STAT6 becomes activated in response to IL-4 and IL-13 and mediates most of the gene expression regulated by these cytokines. By direct interaction with specific parts of its transactivation domain, STAT6 recruits the co-activators p300/CBP and NCoA1 (also called steroid receptor coactivator-1, SRC-1), which are essential for transcriptional activation. In particular, the interaction between STAT6 and NCoA1 is modulated by a short region of the transactivation domain that includes the motif LXXLL (where L is leucine and X is any amino acid). Here, we report the structural characterization of the complex between a STAT6-derived peptide encompassing the region from Gly783 to Gly814 and the NCoA1 PAS-B domain257–385 using NMR and X-ray crystallography.

In this crystal structure the residues located in the N-terminal part (Gly783 - Pro793) are not ordered indicating that this region is too dynamic to be resolved in the crystal. Nevertheless, the new X-ray structure of the complex clarifies the structural role of Leu794 whose side chain fits into a deep pocket on the cofactor surface formed by Phe314, Phe300 and Ala310. Yet, there is no interaction visible between the residues N-terminal of Leu794 in the crystal structure. Therefore, we decided to perform a structural characterization of the NCoA1257–385/STAT6783–814 complex by NMR. Importantly, the interaction between the NCoA1 PAS-B domain and STAT6783–814 is further stabilized by the interaction of STAT6 Leu794 with a shallow hydrophobic indentation constituted by the PAS-B domain residues Phe314, Phe300 and Ala310, seen also in the X-ray structure and in agreement with the alanine scanning mutagenesis data where F794A reduced the affinity about 50-fold. In addition, the two isoleucine residues (Ile786, Ile790) located in the N-terminal part of the STAT6 peptide bind into a shallow hydrophobic pocket on the surface of the PAS-B domain formed by Phe314, Met318, Leu346, Pro356 and Ile358. The NMR structure of the NCoA1257–385/STAT6783–814 complex indicates that the coactivator recognition mechanism by STAT6 occurs by the formation of a partially ordered complex in which two α-helical regions (Ile786-Ile790 and Glu799-Glu808) are connected by a linker that adopts an extended, albeit dynamic, conformation. This dynamics in the linker may act more strongly onto the N-terminal region of the STAT6783–814 peptide that has fewer interactions with the NcoA1 PAS-B domain than the C-terminal region, ultimately rendering residues 783–793 disordered in the X-ray structure. Thus despite the invisibility of the peptide N-terminal to Leu794 in the X-ray structure, the complex formation between the NCoA1 PAS-B domain and STAT6783–814 is well defined by specific interactions in solution.

> GHMTGVESFMTKQDTTGKIISIDTSSLRAAGRTGWEDLVRKCIYAFFQPQGREPSYARQLFQEVMTRGTASSPSYRFILNDGTMLSAHTRCKLCYPQSPDMQPFIMGIHIIDREHSGLSPQDDTNSGMSIPR;> GTWIGEDIFPPLLPPTEQDLTKLLLEGQGESG> PRVYETELLVLRFREFGVKDNHNHPINLHSLRSKSLIRAQGKKLDLHNRVFLRRNVRAVK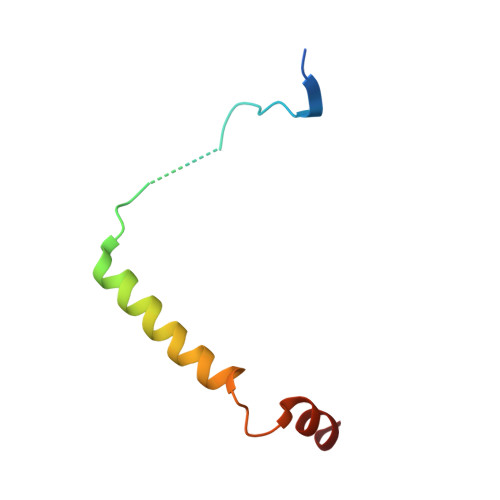M>[4x]MTTSHGLIESQLSYYRARASEYDAT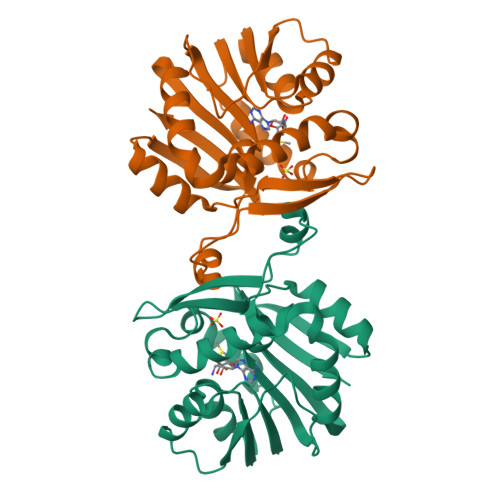FVPYMDSAAPAALERLRAGNIRGDVLELASGTGYWTRHLSGLADRVTALDGSAEMIAEAGRHGLDNVEFRQQDLFDWTPDRQWDAVFFAHWLAHVPDDRFEAFWESVRSAVAPGGVVEFVDVTDHERRLEQQDDSEPEVAVRRTLQDGRSFRIVKVFRSPAELTERLTALGWSCSVDEVHPGFLYATCRPGPR> MDLRRRPPKPPVTNNNNSNGSFRSYQPRTSDDDHRRRATTIAPPPKASDALPLPLYLTNAVFFTLFFSVAYYLLHRWRDKIRYNTPLHVVTITELGAIIALIASFIYLLGFFGIDFVQSFISRASGDAWDLADTIDDDDHRLVTCSPPTPIVSVAKLPNPEPIVTESLPEEDEEIVKSVIDGVIPSYSLESRLGDCKRAASIRREALQRVTGRSIEGLPLDGFDYESILGQCCEMPVGYIQIPVGIAGPLLLDGYEYSVPMATTEGCLVASTNRGCKAMFISGGATSTVLKDGMTRAPVVRFASARRASELKFFLENPENFDTLAVVFNRSSRFARLQSVKCTIAGKNAYVRFCCSTGDAMGMNMVSKGVQNVLEYLTDDFPDMDVIGISGNFCSDKKPAAVNWIEGRGKSVVCEAVIRGEIVNKVLKTSVAALVELNMLKNLAGSAVAGSLGGFNAHASNIVSAVFIATGQDPAQNVESSQCITMMEAINDGKDIHISVTMPSIEVGTVGGG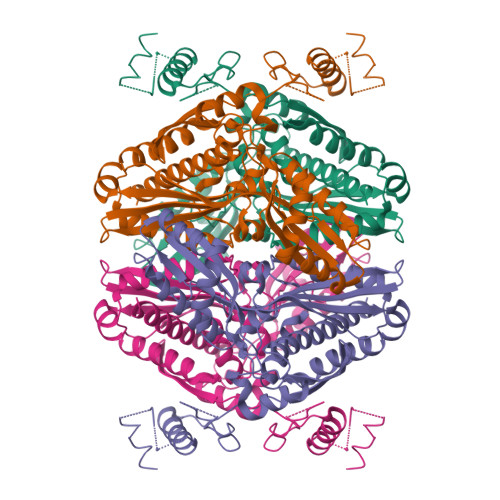TQLASQSACLNLLGVKGASTESPGMNARRLATIVAGAVLAGELSLMSAIAAGQLVRSHMKYNRSSRDISGATTTTTTTT> MSLMLSHNPIVEPFALAHATIVTGDKAGTILRNMTIVVGADGRIEQVAPSIETSIPAEYHYLDGTGKIVMPGLINAHTHLFSQGKPLNPKLATPKGQRMVATFAHSPLGKPYMAATVKHNATTLLESGVTTIRTLGDVGYEVVTLRDQIDAGQILGPRILASGPLMAIPEGHGAPLIALTSGTPEEARTAVAQNLK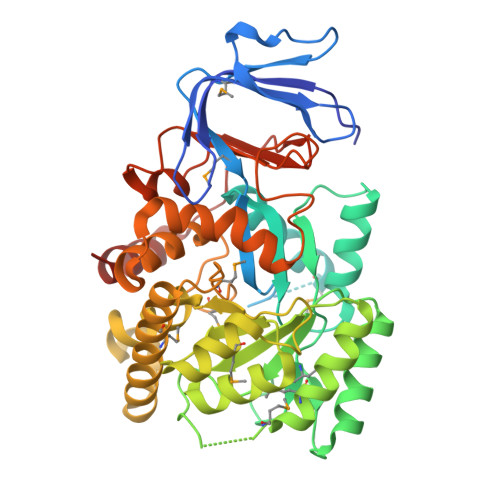AGVNAIKIAATGGVTDAQEIGEAGSPQMSVEQMRAICDEAHQYGVIVGAHAQSPEGVRRSLLAGVDTIEHGSVLDDELIGMFRHNPNALRGYSALIPTLSAGLPLTLLGQDVTGITDIQLENSKNVVGGMVSGARQAHEAGLMIGVGTDTGMTFVPQYATWRELELLVAYAGFSPAEALHAATAVNASILGVDAETGSLEVGKSADLLVLNANPLDDLRALEHPALVIAAGHPVWRPGPKRFADIDALLDEAYAEGHHHHHH>[2x]GTAPKSRNLFERNPNKELKPGENSPRQTPIFDPTVHWLFTTCGASGPHGPTQAQCNNAYQNSNLSVEVGSEGPLKGIQIWKVPATDTYSISGYGAAGGKGGKNTMMRSHGVSVLGIFNLEKDDMLYILVGQQGEDACPSTNQLIQKVCIGENNVIEEEIRVNRSVHEWAGGGGGGGGATYVFKMKDGVPVPLIIAAGGGGRAYGAKTDTFHPERLENNSSVLGLNGNSGAAGGGGGWNDNTSLLWAGKSLQEGATGGHSCPQAMKKWGWETRGGFGGGGGGCSSGGGGGGYIGGNAASNNDPEMDGEDGVSFISPLGILYTPALKVMEGHGEVNIKHYLNCSHCEVDECHMDPESHKVICFCDHGTVLAEDGVSCIVSP;> GAEPREPADGQALLRLVVELVQELRKHHSAEHKGLQLLGRDYALGRAEAAGLGPSPEQRVEIVPRDLRMKDKFLKHLTGPLYFSPKCSKHF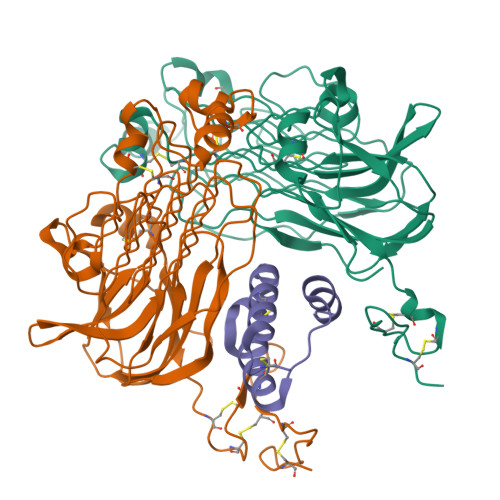HRLYHNTRDCTIPAYYKRCARLLTRLAVSPVCMEDKQ>[2x]GSHMCLVCSDEASGCHYGVLTCGSCKVFFKRAVEGQHNYLCAGRNDCIIDKIRRKNCP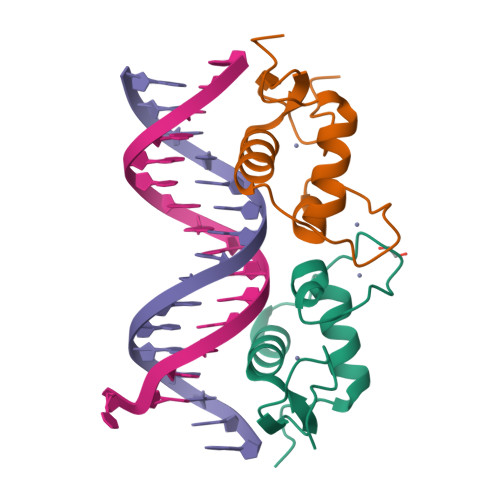ACRYRKCLQAGMNLEARKTKKKIKGIQQATAG>[4x]SANEDMPVERILEAELAVEPKTETYVEANMGLNPSSPNDPVTNICQAADKQLFTLVEWAKRIPHFSELPLDDQVILLRAGWNELLIASFSHRSIAVKDGILLATGLHVHRNSAHSAGV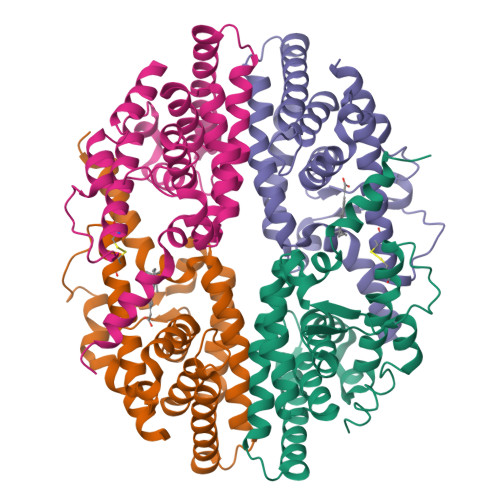GAIFDRVLTELVSKMRDMQMDKTELGCLRAIVLFNPDSKGLSNPAEVEALREKVYASLEAYCKHKYPEQPGRFAKLLLRLPALRSIGLKCLEHLFFFKLIGDTPIDTFLMEMLEAPHQMT4-{8-amino-3-[(6R,8aS)-3-oxooctahydroindolizin-6-yl]imidazo[1,5-a]pyrazin-1-yl}-3-(cyclopropyloxy)-N-[4-(trifluoromethyl)pyridin-2-yl]benzamide | 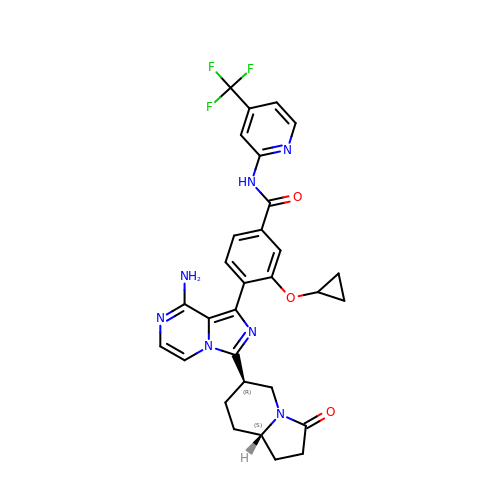C30 H28 F3 N7 O3 | WMMNTQFZCHUZSM-MJGOQNOKSA-N(+)-alpha-Pinene | C10 H16 | 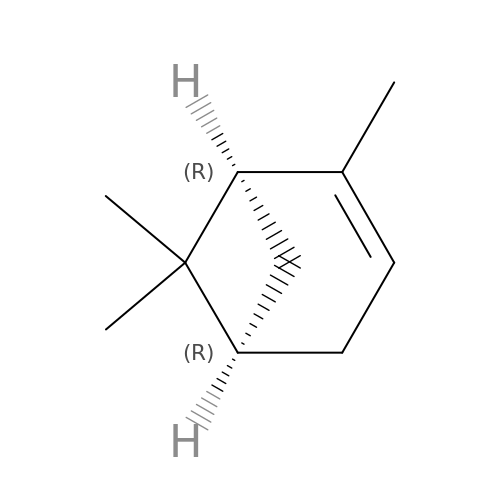GRWFGVWFFZKLTI-RKDXNWHRSA-N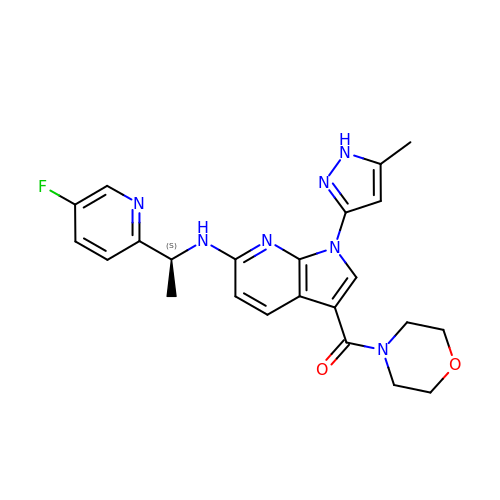[6-{[(1S)-1-(5-fluoropyridin-2-yl)ethyl]amino}-1-(5-methyl-1H-pyrazol-3-yl)-1H-pyrrolo[2,3-b]pyridin-3-yl](morpholin-4-yl)methanone | C23 H24 F N7 O2 | UYIANZRYPSGDFM-HNNXBMFYSA-N>[12x]XGEIAQAFKEIAK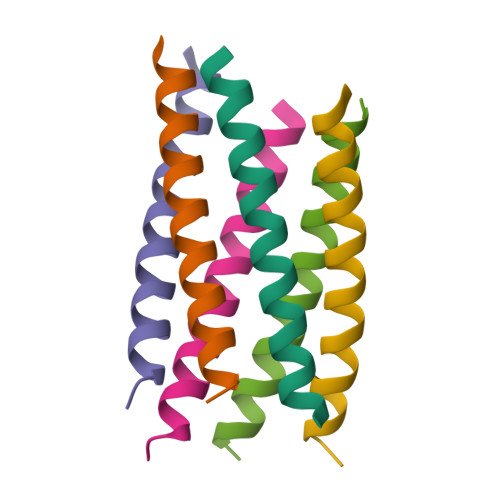AFKEIAWAFKEIAQAFKGX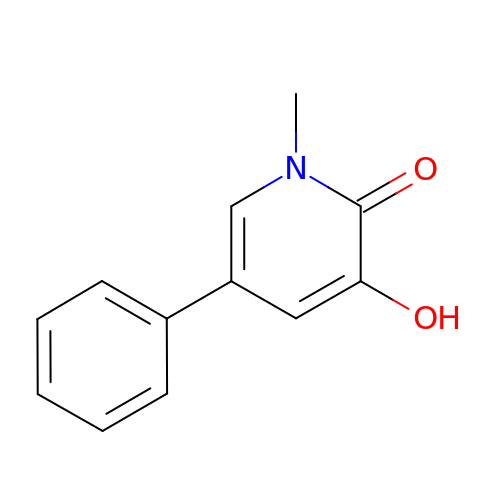1-methyl-3-oxidanyl-5-phenyl-pyridin-2-one | C12 H11 N O2 | NDVZUSAEFIBAFV-UHFFFAOYSA-N>GSHMAATYKKPSDAELKRTLTEEQYQVTQNSATEYAFSHEYDHLFKPGIYVDVVSGEPLFSSADKYDSGCGWPSFTRPIDAKSVTEHDDFSFNMRRTEVRSRAADSHLGHVFPDGPRDKGGLRYCINGAS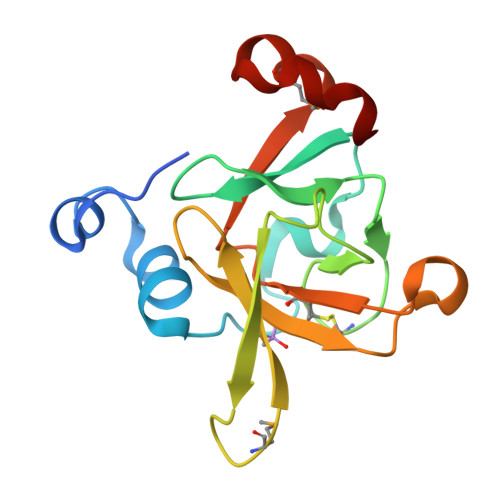LKFIPLEQMDAAGYGALKGEVK[2x]> MGNEQDSEIYRFDQFMNTDDYIWVFNTTQEGPKECEKDKKHNMTNDKIIFVRSHQEETKIVNETIIG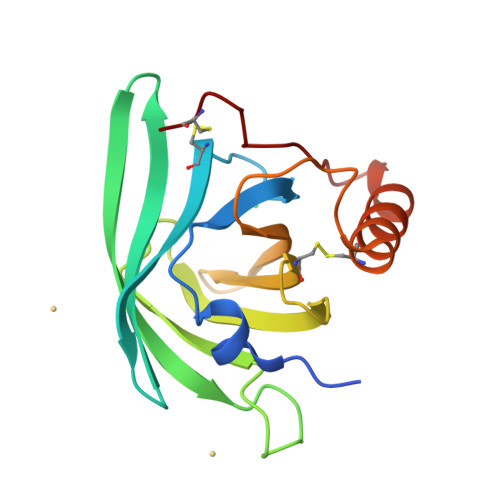DFFHYSDNKSVYDGIYISGDKREVHAEHLYYSSEDMICGLVQVFARQTDAWTELRVRGRRSYKSLDEVCRTQYEKYVEAIKHTKTSTSPYRDDCQ>VLSGCSNNVSSIKIDRFNNISAVNGPGEEDTWASAQKQGVGTANNYVSKVWFTLANGAISEVYYPTIDTADVKEIKFIVTDGKSFVPDETKDAISKVEKFTDKSLGYKLVNTDKKG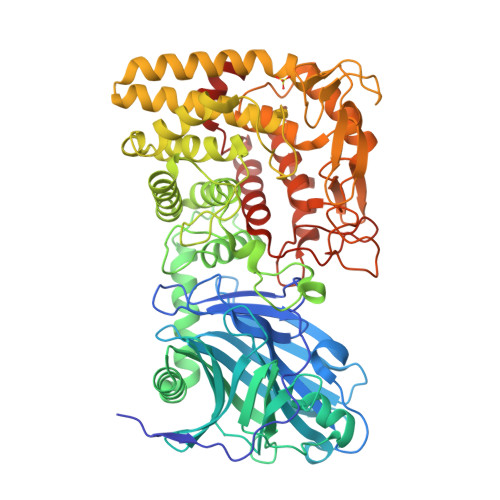RYRITKDIFTDVKRNSLIMKAKFEALEGSIHDYKLYLAYDPHIKNQGSYNEGYVIKANNNEMLMAKRDNVYTALSSNIGWKGYSIGYYKVNDIMTDLDENKQMTKHYDSARGNIIEGAEIDLTKNSEFEIVLSFGQSDSEAAKTALETLGEDYNNLKNNYIDEWTKYCNTLNNFNGKANSLYYNSMMILKASEDKTNKGAYIASLSIPWGDGQRDDNTGGYHLVWSRDLYHVANAFIAAGDVDSANRSLDYLAKVVKDNGMIPQNTWISGKPYWTGIQLDEQADPIILSYRLKRYDLYDSLVKPLADFIIKIGPKTGQERWEEIGGYSPATMAAEVAGLTCAAYIAEQNKDYESAQKYQEKADNWQKLIDNLTYTENGPLGNGQYYIRIAGLSDPDADFMINIANGGGVYDQKEIVDPSFLELVRLGVKSADDPKILNTLKVVDSTIKVDTPKGPSWYRYNHDGYGEPSKTELYHGAGKGRLWPLLTGERGMYEIAAGKDATPYVKAMEKFANEGGIISEQVWEDTGLPTDSASPLNWAHAEYVILFASNIEHKVLDMPDIVYKRYVA[2x]>[8x]MVQASGHRRSTRGSKMVSWSVIAKIQEILQRKMVREFLAEFMSTYVMMVFGLGSVAHMVLNKKYGSYLGVNLGFGFGVTMGVHVAGRISGAHMNAAVTFANCALGRVPWRKFPVYVLGQFLGSFLAAATIYSLFYTAILHFSGGQLMVTGPVATAGIFATYLPDHMTLWRGFLNEAWLTGMLQLCLFAITDQENNPALPGTEALVIGILVVIIGVSLGMNTGYAINPSRDLPPRIFTFIAGWGKQVFSN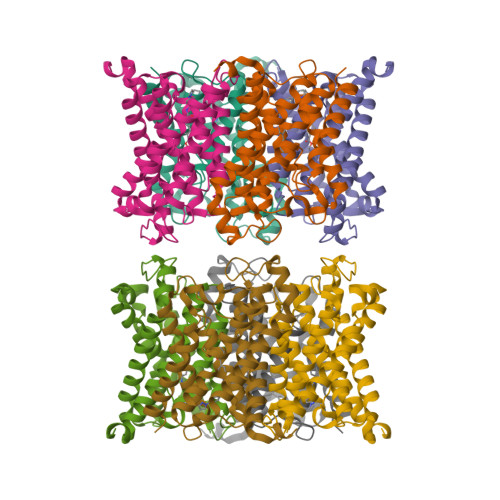GENWWWVPVVAPLLGAYLGGIIYLVFIGSTIPREPLKLEDSVAYEDHGITVLPKMGSHEPTISPLTPVSVSPANRSSVHPAPPLHESMALEHF>MENSLFNQEVQIPLTESYCGPCPKNWICYKNNCYQFFDESKNWYESQASCMSQNASLLKVYSKEDQDLLKLVKSYHWMGLVHIPTNGSWQWEDGSILSPNLLTIIEMQKGDCALYASSFKGYIENCSTPNTYICMQRTV[2x];> MEPHSLRYNLTVLMWDGSVQSGFLTEVHLDGQPFLRCDRQKCRAKPQGQWAEDVLGNKTWDRETRDLTGNGKDLRMTLAHIKDQKEGLHSLQEIRVCEIHEDNSTRSSIHFYYDGELFLSGNLETKEWTMPQSSRAQTLAMNVRNFWKEDAMKTKTHWHAMHADCLQELRRYLK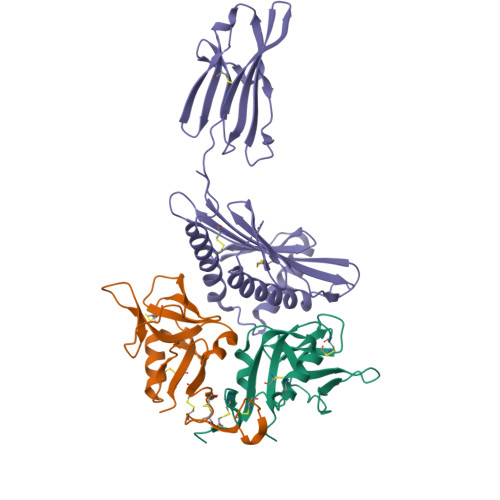SGVVLRRTVPPMVNVTRSEASEGNITVTCRASGFYPWNITLSWRQDGVSLSHDTQQWGDVLPDGNGTYQTWVATRICQGEEQRFTCYMEHSGNHSTHPVPS> PISPIETVPVKLKPGMDGPKVKQWPLTEEKIKALVEICTEMEKEGKISKIGPENPYNTPVFAIKKKDSTKWRKLVDFRELNKRTQDFWEVQLGIPHPAGLKKKKSVTVLDVGDAYFSVPLDEDFRKYTAFTIPSINNETPGIRYQYNVLPQGWKGSPAIFQSSMTKILEPFKKQNPDIVIYQYMDDLYVGSDLEIGQHRTKIEELRQHLLRWGLTTPD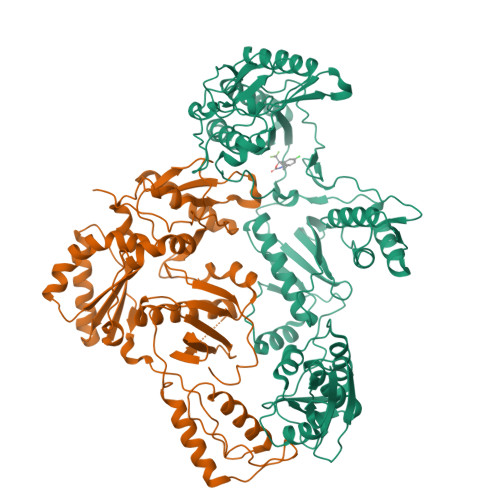KKHQKEPPFLWMGYELHPDKWTVQPIVLPEKDSWTVNDIQKLVGKLNWASQIYPGIKVRQLCKLLRGTKALTEVIPLTEEAELELAENREILKEPVHGVYYDPSKDLIAEIQKQGQGQWTYQIYQEPFKNLKTGKYARMRGAHTNDVKQLTEAVQKITTESIVIWGKTPKFKLPIQKETWETWWTEYWQATWIPEWEFVNTPPLVKLWYQLEKEPIVGAETFYVDGAANRETKLGKAGYVTNKGRQKVVPLTNTTNQKTQLQAIYLALQDSGLEVNIVTDSQYALGIIQAQPDKSESELVNQIIEQLIKKEKVYLAWVPAHKGIGGNEQVDKLVSAGIRKIL;> PISPIETVPVKLKPGMDGPKVKQWPLTEEKIKALVEICTEMEKEGKISKIGPENPYNTPVFAIKKKDSTKWRKLVDFRELNKRTQDFWEVQLGIPHPAGLKKKKSVTVLDVGDAYFSVPLDEDFRKYTAFTIPSINNETPGIRYQYNVLPQGWKGSPAIFQSSMTKILEPFKKQNPDIVIYQYMDDLYVGSDLEIGQHRTKIEELRQHLLRWGLTTPDKKHQKEPPFLWMGYELHPDKWTVQPIVLPEKDSWTVNDIQKLVGKLNWASQIYPGIKVRQLCKLLRGTKALTEVIPLTEEAELELAENREILKEPVHGVYYDPSKDLIAEIQKQGQGQWTYQIYQEPFKNLKTGKYARMRGAHTNDVKQLTEAVQKITTESIVIWGKTPKFKLPIQKETWETWWTEYWQATWIPEWEFVNTPPLVKLWY> SNSGTEQQNPRGSSLLTDPESITKSDPYNPNISLLISGEVFTNFRNLIKRVNFRKATTLNGKRISDTFDINSLIEAPRLDIAQYVDTETKEAKYGFSYFWSAPTTLNIVAEMYALYRGGVRVKVVTEKGVDFVRATVSPQQTYGSDVAPTTHISTPLAIEQIPIKGVAEFQIPYYAPCLSSSFRANSETFYYSSGRNNLDIATSPPSINRYYAVGAGDDMDFSIFIGTPPCIHASQTAQFTKIKQGKVYDLRYDQYDPFREVQDGTAFLNARSIEDSDLL;> MAEQINENYENKQQLVEQTEITTFENDLIVLEDGPQMEESLPFAFHGQHTDNRQHTVVNFLQRPQVIFDSSWASDVPRNKQFMDSIMIPDDIISFPMFAEKLKGFSSLRATAVITVQFQTQPFQAGRVMLGSFPLPTLNPTRVKFATNHVSRLMLLNHVQCDIAKETEVSLRIPFVSPYNSYDLVSKRFPWAKVVGLVYSPLTTTIPVDFIVYGHFEDVELGCPTSGMLAQ;> SKPLLPIANPTVLRPANTFAITDTNDMSHSLALSNDTNVPFVKALDGSGLDEMSFDYLKKIPQFIQSKFFTTTTKPQEVLFQTKVMPHYFVPGGDVTVAMDKDITRTIWQPSHLAYITSMFKYWTGSLVYTFKFVKTDYHSGRVEVSFHPFSDYTTGTYSDYTYRIIVDLREKSEFSVTIPFISPVPYKRISRPDWDKPYSKYAHASTGTLVLKALTSLK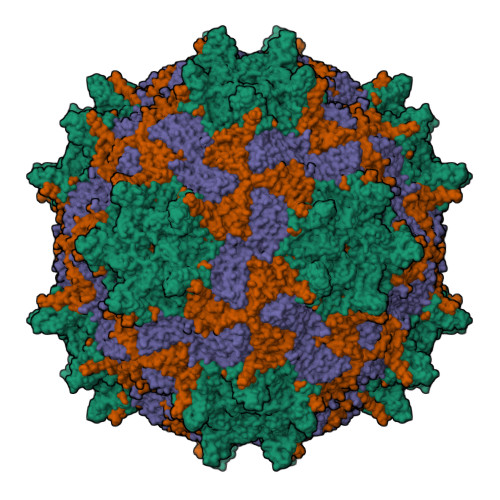ATNTVVSNSVEILIEVNAGDDFNVIAPIENIFFPFSLSPGRKGMVAQ> MKDLVDTTEMYLRTIYELEEEGVTPLRARIAERLEQSGPTVSQTVARMERDGLVVVASDRSLQMTPTGRTLATAVMRKARLAERLLTDIIGLDIN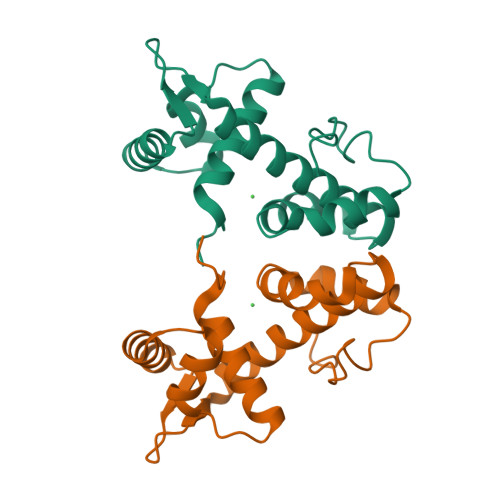KVHDEADRWEHVMSDEVERRLVKVLKDVSRSPFGNPIPGLDELG>[8x]MTVQTSKNPQVDIAEDNAFFPSEYSLSQYTSPVSDLDGVDYPKPYRGKHKILVIAADERYLPTDNGKLFSTGNHPIETLLPLYHLHAAGFEFEVATISGLMTKFEYWAMPHKDEKVMPFFEQHKSLFRNPKKLADVVASLNADSEYAAIFVPGGHGALIGLPESQDVAAALQWAIKNDRFVISLCHGPAAFLALRHGDNPLNGYSICAFPD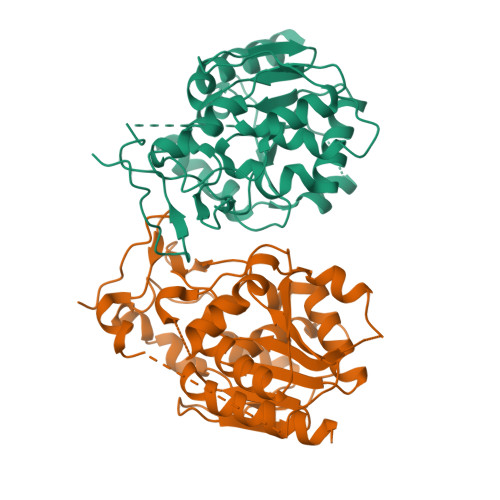AADKQTPEIGYMPGHLTWYFGEELKKMGMNIINDDITGRVHKDRKLLTGDSPFAANALGKLAAQEMLAAYAG Rspo (R-spondin, also roof plate-specific spondin) proteins are evolutionarily conserved from fish to humans and have well-documented roles in a broad range of developmental and physiological processes resulting from enhancement of canonical and non-canonical Wnt signalling. ZNRF3/RNF43 specifically targets these Wnt receptors for ubiquitination and turnover, hence reducing Wnt signalling responses. Direct extracellular interaction with Rspo proteins inhibits ZNRF3/RNF43 activity. Here we report a molecular level analysis of the ZNRF3/RNF43 ectodomain structure and its interactions with Rspo proteins.

By using a combination of heavy atom and molecular-replacement-based phasing strategies, we determined multiple crystal structures for Xenopus (x) Rspo2Fu1–Fu2 (highest resolution 2.2 Å), xZNRF3ecto, zebrafish (z) ZNRF3ecto and mouse (m) ZNRF3ecto, (highest resolutions 2.4, 1.6 and 2.0 Å, respectively), plus complexes comprising xZNRF3ecto–xRspo2Fu1–Fu2, mZNRF3ecto–mRspo2Fu1–Fu2, mZNRF3ecto–xRspo2Fu1–Fu2 and xRNF4F3ecto–xRspo2Fu1–Fu2 (at 2.1, 2.8, 2.4 and 2.7 Å, respectively). The crystal structures of the ZNRF3ecto–Rspo2Fu1–Fu2 and RNF43ecto–Rspo2Fu1–Fu2 complexes revealed a 1:1 interaction between Fu1 of the Rspo2Fu1–Fu2 and a single ZNRF3ecto or RNF43ecto chain. The first, extensive, area of interaction involves hydrophobic interactions interspersed with hydrophilic (complementarily charged) patches contributed by the first two β-hairpins of the Rspo Fu1 and the region immediately carboxy-terminal to the β3 strand of ZNRF3ecto. The Met-finger at the tip of the second β-hairpin of Fu1 nestles into a pocket formed between the β3 strand and the αC–β7 loop of the ZNRF3ecto, which is lined with hydrophobic residues (I95, I191, V192, A198). The acidic region of the β3–β4 loop (immediately adjacent to C104 of the disulphide bridge) becomes more ordered in the ligand-bound ZNRF3ecto structures, probably as a result of electrostatic interactions with a positively charged patch on Rspo Fu1. For all ZNRF3ecto–Rspo2Fu1–Fu2 complex structures we determined (from five different combinations of species and crystal forms), the dimer found in most of the unliganded ZNRF3ecto crystal structures reoccurs. The overall assembly thus comprises a 2:2 complex of ZNRF3ecto–Rspo2Fu1–Fu2. The 2:2 complex resembles a crab with the ZNRF3ecto dimer forming the body from which the two Rspo2Fu1–Fu2 ligands diverge, without interacting with each other, as the pincers. Notably, the β1–β2 hairpin shows less conformational variation in the liganded ZNRF3ecto dimer structures, always maintaining a tight embrace, consistent with the Rspo2Fu1–Fu2 interactions contributing an indirect stabilizing effect on the dimer via the β3–β4 loop. For the ligand–receptor mode, our data define a generic architecture for the interaction between the Rspo ligands, and the ZNRF3 and RNF43 transmembrane E3 ubiquitin ligases that is conserved across evolution from fish to human.

>[2x]ETGKETAFVEVVLFESSPSGDYTTHTTGLTGRFSRAGAMLSAEGEIVQMHPLGLCNNNDEEDLYEYGWVGVVKLEQPELDPKPCLTVLGKAKRAVQRGATAVIFDVSENPEAIDQLNQGSEDPLKRPVVYVKGADAIKLMNIVNKQKVARARIQHLGTKHHHHHH;>ETGNPICKGCLSCSKDNGCSRCQQKLFFFLRREGMRQYGECLHSCPSGYYGHRAPDMNRCARCRIENCDSCFSKDFCTKCKVGFYLHRGRCFDECPDGFAPLDETMECVEGTHHHHHHHHHH[2x]> GPLGSMSMAMSQSNRELVVDFLSYKLSQKGYSWSQFSDVEENRTEA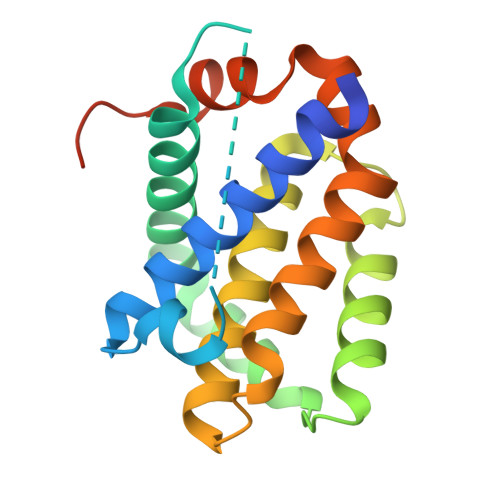PEGTESEAVKQALREAGDEFELRYRRAFSDLTSQLHITPGTAYQSFEQVVNELFRDGVNWGRIVAFFSFGGALCVESVDKEMQVLVSRIAAWMATYLNDHLEPWIQENGGWDTFVELYGNNAAAESRKGQERLE>SMPALSSQSKLSQAAQETKQKLTSCLARRYNAEQKLLDLSALGTDETLSSLGSFNNQSLAEKSFKALMHLVSNEYKDPEQKNEAIQAVSLARNDILDVGQVYSLAVTLPRLRRLDLSGNNLENLSKISKWQQEFRFLEELHLTGNPVTTLPNYATEIKKWFPSLQILDGQQIRTPQEAAESLKSSFPTPLPQLPSNVRDGENNVASTFLQAFFQLWDHDRLTLIPQFYDSETTFSVVFATDSPQDPASSSCSKFSRNLNILSPRHPSTLQRLFVGSNLIA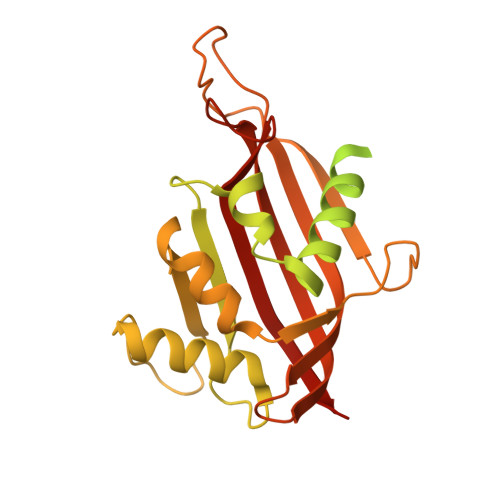DLWKVLPATRHPSLDQTSQWLIDCHTFPHLADPTGMAPYAMGLMINVNGQCEEADISQNLYGTRTFSRCFILGPSKPGAPHPYRVLSDQLTLHTWKPQPAPQVGTV[4x]>MRYLTAGESHGPRLTAIIEGIPAGLPLTAEDINEDLRRRQGGYGRGGRMKIENDQVVFTSGVRHGKTTGAPITMDVINKDHQKWLDIMSAEDIEDRLKSKRKITHPRP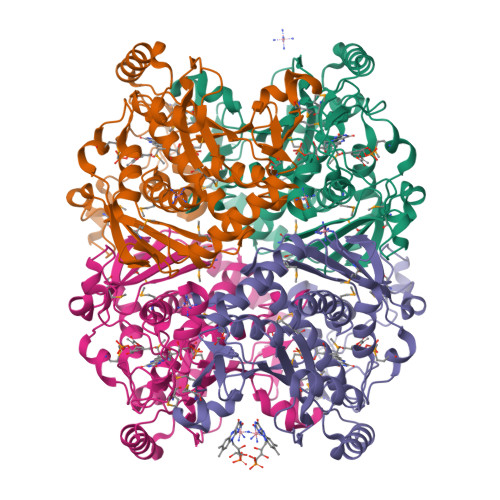GHADLVGGIKYRFDDLRNSLERSSARETTMRVAVGAVAKRLLAELDMEIANHVVVFGGKEIDVPENLTVAEIKQRAAQSEVSIVNQEREQEIKDYIDQIKRDGDTIGGVVETVVGGVPVGLGSYVQWDRKLDARLAQAVVSINAFKGVEFGLGFEAGYRKGSQVMDEILWSKEDGYTRRTNNLGGFEGGMTNGQPIVVRGVMKPIPTLYKPLMSVDIETHEPYKATVERSDPTALPAAGMVMEAVVATVLAQEILEKFSSDNLEELKEAVAKHRDYTKNY[4x]> MEYTTLAVLAGLPEDPHGAVGLPIYAVAAYGFKTLEEGQERFATGEGYVYARQKDPTAKALEERLKALEGALEAVVLASGQAATFAALLALLRPGDEVVAAKGLFGQTIGLFGQVLSLMGVTVRYVDPEPEAVREALSAKTRAVFVETVANPALLVPDLEALATLAEEAGVALVVDNTFGAAGALCRPLAWGAHVVVESLT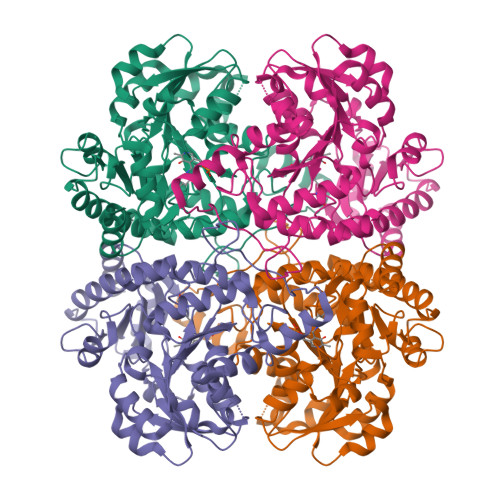KWASGHGSVLGGAVLSRETELWRNYPQFLQPDLKGQIPWEALRARCFPERVRTLGLSLCGMALSPFNAYLLFQGLETVALRVARMSETARFLAERLQGHPKVKALRYPGLPEDPAHRNARKYLASGGPILTLDLGDLERASRFLGAIRLLKAANLGDARTLLVHPWTTTHSRLKEEARLQAGVTPGLVRVSVGLEDPLDLLALFEEALEAV2-(3-chlorophenoxy)-4-{(1R)-3-methyl-1-[(3S)-3-(5-methyl-2,4-dioxo-3,4-dihydropyrimidin-1(2H)-yl)piperidin-1-yl]butyl}benzoic 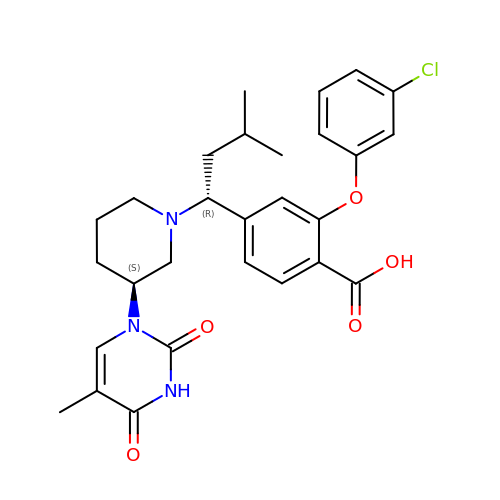acid | C28 H32 Cl N3 O5 | DUMBOKZAFBZKLT-XUZZJYLKSA-N IMIDAZO[2,1-A]ISOQUINOLINE-2-CARBOHYDRAZIDE | C12 H10 N4 O | 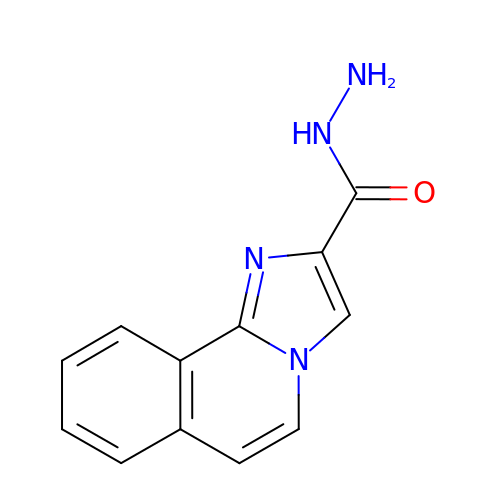WSNWYZBDIKCPIG-UHFFFAOYSA-N> GFTDYKVADITLAAWGRRELIIAESEMPALMGLRRKYAGQQPLKGAKILGCIHMTIQTGVL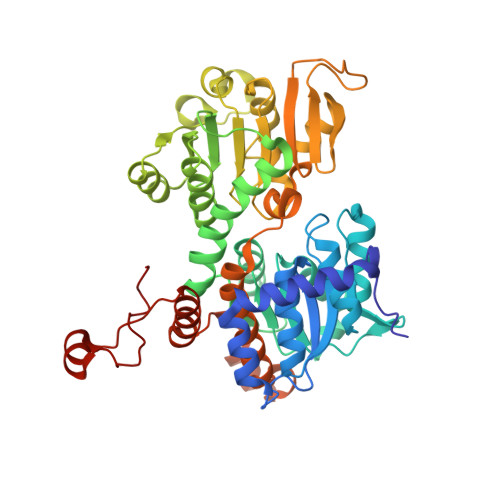IETLVALGAEVRWSSCNIFSTQDQAAAAIAAAGIPVFAWKGETEEEYEWCIEQTILKDGQPWDANMVLDDGGDLTEILHKKYPQMLERIHGITEETTTGVHRLLDMLKNGTLKVPAINVNDSVTKSKNDNKYGCRHSLNDAIKRGTDHLLSGKQALVIGYGDVGKGSSQSLRQEGMIVKVAEVDPICAMQACMDGFEVVSPYKNGINDGTEASIDAALLGKIDLIVTTTGNVNVCDANMLKALKKRAVVCNIGHFDNEIDTAFMRKNWAWEEVKPQVHKIHRTGKDGFDAHNDDYLILLAEGRLVNLGNATGHPSRIMDGSFANQVLAQIHLFEQKYADLPAAEKAKRLSVEVLPKKLDEEVALEMVKGFGGVVTQLTPKQAEYIGVSVEGPFKPDTYRY> GSSMGSLNQDATILRQAKLGLSDPAQSLSSWSDNNDVTPCKWLGVSCDATSNVVSVDLSSFMLVGPFPSILCHLPSLHSLSLYNNSIN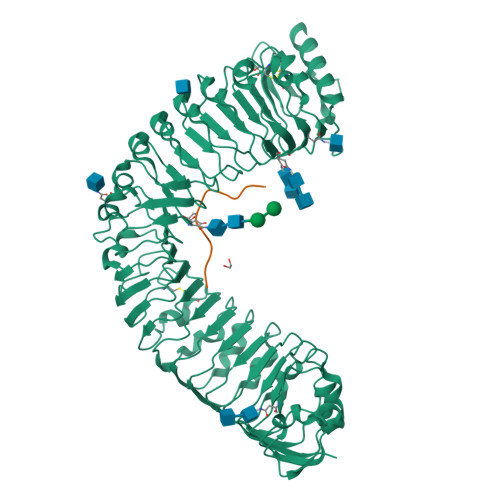GSLSADDFDTCHNLISLDLSENLLVGSIPKSLPFNLPNLKFLEISGNNLSDTIPSSFGEFRKLESLNLAGNFLSGTIPASLGNVTTLKELKLAYNLFSPSQIPSQLGNLTELQVLWLAGCNLVGPIPPSLSRLTSLVNLDLTFNQLTGSIPSWITQLKTVEQIELFNNSFSGELPESMGNMTTLKRFDASMNKLTGKIPDNLNLLNLESLNLFENMLEGPLPESITRSKTLSELKLFNNRLTGVLPSQLGANSPLQYVDLSYNRFSGEIPANVCGEGKLEYLILIDNSFSGEISNNLGKCKSLTRVRLSNNKLSGQIPHGFWGLPRLSLLELSDNSFTGSIPKTIIGAKNLSNLRISKNRFSGSIPNEIGSLNGIIEISGAENDFSGEIPESLVKLKQLSRLDLSKNQLSGEIPRELRGWKNLNELNLANNHLSGEIPKEVGILPVLNYLDLSSNQFSGEIPLELQNLKLNVLNLSYNHLSGKIPPLYANKIYAHDFIGNPGLCVDLDGLCRKITRSKLEGSENLYFQ;> LVPPSGPSMRHN>[4x]MSSATPDPAEILTARKAVGLSQTAAAALVHSS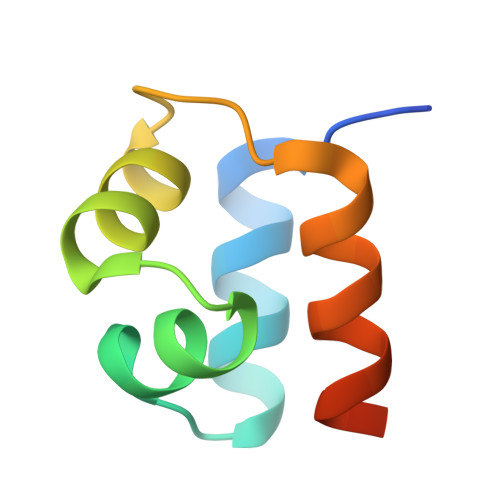LRTWQQWEAGDRRMHPGLWELFLLKTQLPSPSS> WGKEGHEIICKIAQTRLDETAAKAVKELLPESAEGDLSSLCLWADRVKFRYHWSSPLHYINTPDACSYQYNRDCKDESGEKGRCVAGAIYNYTTQLLSYKTAASSQSEYNLTEALLFVSHFMGDIHQPLHVSYASDKGGNTIEVHWYTRKANLHHIWDSNIIETAEADLYNSALEGMVDALKKNITTEWADQVKRWETCTKKTACPDIYASEGIQAACDWAYKGVTEGDTLEDEYFYSRLPIVYQRLAQGGVRLAATLNRIFGHHHHHH

AtBFN2 (also called ENDO2) is a 34.5 kDa glycoprotein (the predicted mass for protein component alone is 30.5 kDa), encoded by the Arabidopsis thaliana At1g68290 gene. AtBFN2 follows the standard glycosylation pattern of plant S1/P1 endonucleases, with three glycosylation sites (Asn91, Asn110, and Asn184). While the P1 nuclease has a higher specificity for RNA over ssDNA, in a previous study we showed that the opposite is true for AtBFN2. Structurally, Zn2+-dependent endonucleases present a unique fold, and are classified into the P1/S1 nuclease family (pfam ID PF02265), itself part of the Phospholipase C (PLC)/P1 nuclease superfamily (pfam ID CL0368).

Finally, we obtained a detailed ssDNA•AtBFN2 co-crystal structure by soaking the crystals with a thiophosphorylated ssDNA analog. In this structure a large secondary ssDNA binding site was observed. A single deoxythymidine monophosphate residue was bound to the active site, in much the same way as has been described for P1 nuclease. The thymine moiety was stacked against Tyr59 and lodged within a pocket comprising the peptide backbones of His130, Lys137, and Gly138, and the side-chains of Tyr59, Asn61, and Leu129. The deoxyribose was bound to Asn140 at the ring oxygen, while the 3′-end was tightly coordinated to Zn2, displacing the Wat3, which was present in the other three structures. Under these conditions, we also found a single sulfate anion within the binding pocket, which had displaced the other waters, including catalytically relevant Wat1. The secondary binding site is completely novel, and much larger than the active site pocket. In it, elements from both the protein and the N-glycan at Asn91 participate in the binding of a dinucleotide composed of one adenosine, and one thymidine. Indeed, GlcNAc1 at Asn91 interacts via its acetyl group with the 3′-end of the thymidine deoxyribose, which also interacts with the backbone of Lys81. The secondary binding site possibly reveals a new and crucial role for glycosylation at Asn91, since GlcNAc1 is an important partner in binding the dinucleotide.>SAKKNEPRFKNGIVAALAGFFILGIGTVGTLWILNSPQRQAAELDSLLGQEKERFQVLPGRDKMLYVAAQNERDTLWARQVLARGDYDKNARVINENEENKRISIWLDTYYPQLAYYRIHFDEPRKPVFWLSRQRNTMSKKELEVLSQKLRALMPYADSVNITLMDDVTAAGQAEAGLKQQALPYSRRNHKGGVTFVIQGALDDVEILRARQFVDSYYRTWGGRYVQFAIELKDDWLKGRSFQYGAEGYIKMSPGHWYFPSPL[24x];>CKDKDLLKGLDQEQANEVIAVLQMHNIEAN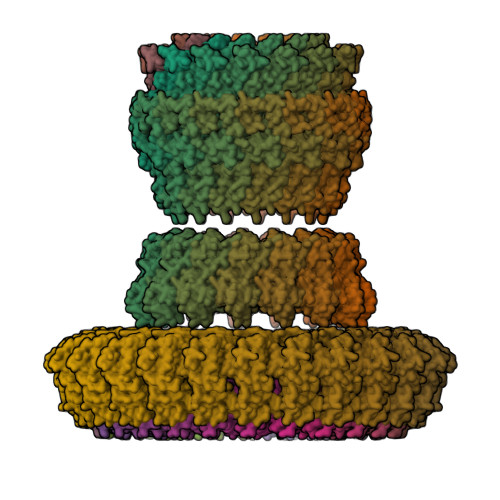KIDSGKLGYSITVAEPDFTAAVYWIKTYQLPPRPRVEIAQMFPADSLVSSPRAEKARLYSAIEQRLEQSLQTMEGVLSARVHISYDIDAGENGRPPKPVHLSALAVYERGSPLAHQISDIKRFLKNSFADVDYDNISVVLSERSDAQLQAPGTPVKRNSFATSWIVLIILLSVMSAGFGVWYYKNHYARNKKGITADDKAKSSNE[24x];>[15x]MKTHILLARVLACAALVLVTPGYSSEKIPVTGSGFVAKDDSLRTFFDAMALQLKEPVIVSKMAARKKITGNFEFHDPNALLEKLSLQLGLIWYFDGQAIYIYDASEMRNAVVSLRNVSLNEFNNFLKRSGLYNKNYPLRGDNRKGTFYVSGPPVYVDMVVNAATMMDKQNDGIELGRQKIGVMRLNNTFVGDRTYNLRDQKMVIPGIATAIERLLQGEEQPLGNIVSSEPPAMPAFSANGEKGKAANYAGGMSLQEALKQNAAAGNIKIVAYPDTNSLLVKGTAEQVHFIEMLVKALDVAKRHVELSLWIVDLNKSDLERLGTSWSGSITIGDKLGVSLNQSSISTLDGSRFIAAVNALEEKKQATVVSRPVLLTQENVPAIFDNNRTFYTKLIGERNVALEHVTYGTMIRVLPRFSADGQIEMSLDIEDGNDKTPQSDTTTSVDALPEVGRTLISTIARVPHGKSLLVGGYTRDANTDTVQSIPFLGKLPLIGSLFRYSSKNKSNVVRVFMIEPKEIVDPLTPDASESVNNILKQSGAWSGDDKLQKWVRVYLDRGQEAIK> GPDSMAEPASVAAES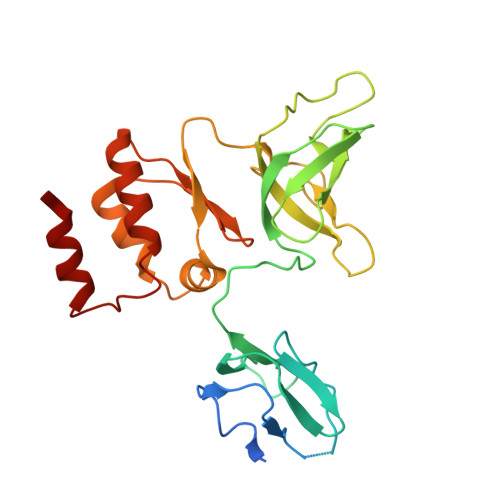LAGSRARAARTVLGQVVLPGEELLLPEQEDAEGPGGAVERPLSLNARACSRVRVVCGPGLRRCGDRLLVTKCGRLRHKEPGSGSGGGVYWVDSQQKRYVPVKGDHVIGIVTAKSGDIFKVDVGGSEPASLSYLSFEGATKRNRPNVQVGDLIYGQFVVANKDMEPEMVCIDSCGRANGMGVIGQDGLLFKVTLGLIRKLLAPDCEIIQEVGKLHPLEIVFGMNGRIWVKAKTIQQTLILANILEACEHMTSDQRKQIFSRLAES> SLTRIDHIGIACHDLDA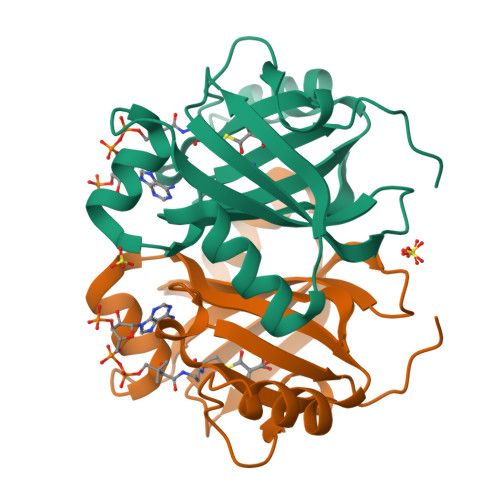TVEFYRATYGFEVFHTEVNEEQGVREAMLKINDTSDGGASYLQLLEPTREDSAVGKWLAKNGEGVHHIAFGTADVDADAADIRDKGVRVLYDEPRRGSMGSRITFLHPKDCHGVLTELVTSAAVESPEH>[2x]MSLQLRLALNQIDSTVGDIAGNAEAILRWTRHSAEQGAHLVAFPEMALTGYPVEDLALRSSFVEASRTALRELAARLAEEGFGELPVLVGYLDRSESAQPKYGQPAGAPRNAAAVLHRGRVALTFAKHHLPNYGVFDEFRYFVPGDTMPIVRLHGVDIALAICEDLWQDGGRVPAARSAGAGLLLSVNASPYERDKDDTRLELVRKRAQEAGCTTAYLAMIGGQDELVFDGDSIVVDRDGEVVARAPQFSEGCVVLDLDLPAAEAEPPTGVVDDGLRIDRLVISE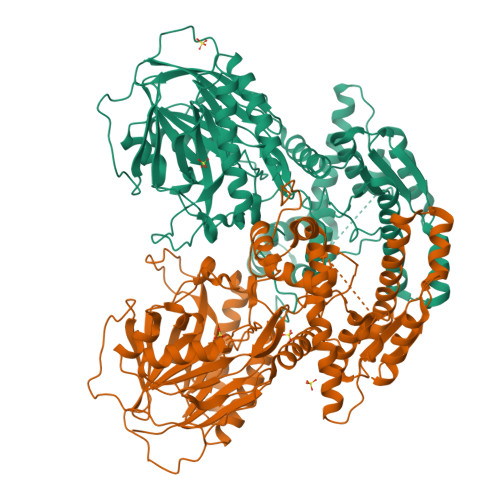EPLPAYEAELAGGYADRLDADEEVYSALVVGLRAYVAKNGFRSVLIGLSGGIDSALVAAIACDALGAQNVYGVSMPSKYSSDHSKGDAAELARRTGLNFRTVSIEPMFDAYMASLGLTGLAEENLQSRLRGTTLMAISNQEGHIVLAPGNKSELAVGYSTLYGDSVGAYGPIKDVYKTSIFRLAEWRNRAAAERGQTPPIPEASITKPPSAELRPGQVDTDSLPDYPVLDAILELYVDRDTGADAIVAAGYDRELVVKTLRMVDTAEYKRRQYPPGTKISAKGFGKDRRLPITNRWREGHHHHHH>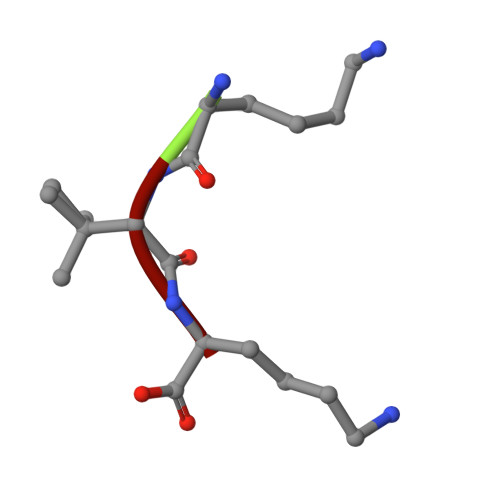 KVK>GSMGLSRVYSKLYKEAEKIKKWKVSTEAELRQKESKLQENRKIIEAQRKAIQELQFGNEKVSLKL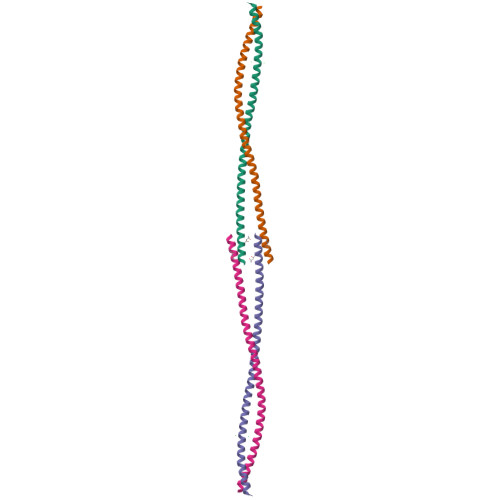EEGIQENKDLIKENNATRHLCNLLKETCARSAEKTKKYEYEREE[2x]>[3x]IQTTAPPVKESSFVEKMKKTGRNIIVFYGSQTGTAEEFANRLSKDAHRYGMRGMSADPEEYDLADLSSLPEIDKSLVVFCMATYGEGDPTDNAQDFYDWLQETDVDLTGVKFAVFGLGNKTYEHFNAMGKYVDQRLEQLGAQRIFELGLGDDDGNLEEDFITWREQFWPAVCEFFGVEASSIRQYELVVHEDMDVAKVYTGEMGRLKSYENQKPPFDAKNPFLAAVTANRKLNQGTERHLMHLELDISDSKIRYESGDHVAVYPANDSALVNQIGEILGADLDVIMSLNNLDEESNKKHPFPCPTTYRTALTYYLDITNPPRTNVLYELAQYASEPSEQEHLHKMAS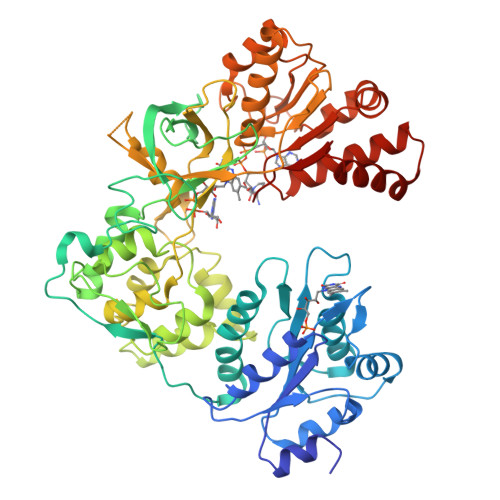SSGEGKELYLSWVVEARRHILAILQDYPSLRPPIDHLCELLPRLQARYYSIASSSKVHPNSVHICAVAVEYEAKSGRVNKGVATSWLRAKEPAGENGGRALVPMFVRKSQFRLPFKSTTPVIMVGPGTGIAPFMGFIQERAWLREQGKEVGETLLYYGCRRSDEDYLYREELARFHKDGALTQLNVAFSREQAHKVYVQHLLKRDREHLWKLIHEGGAHIYVCGDARNMAKDVQNTFYDIVAEFGPMEHTQAVDYVKKLMTKGRYSLDVWS> LKCNQLIPPFYKTCAAGK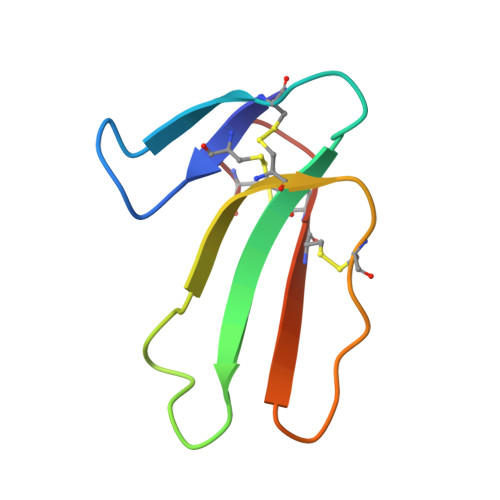NLCYKMFMVAAPKVPVKRGCIDVCPKSSLLVKYVCCNTDRCN> MYYGISQFSEAYNKILRNSSSHSSCQLVIFVSCLNIDALCATKMLSLLFKKQLVQSQIVPIFGYSELRRHYSQLDDNINSLLLVGFGGVIDLEAFLEIDPQEYVIDTDEKSGEQSFRRDIYVLDAHRPWNLDNIFGSQIIQCFDDGTVDDTLGEQKEAYYKLLELDEESGDDELSGDENDNNGGDDEATDADEVTDEDEEDEDETISNKRGNSSIGPNDLSKRKQRKKQIHEYEGVLEEYYSQGTTVVNSISAQIYSLLSAIGETNLSNLWLNILGTTSLDIAYAQVYNRLYPLLQDEV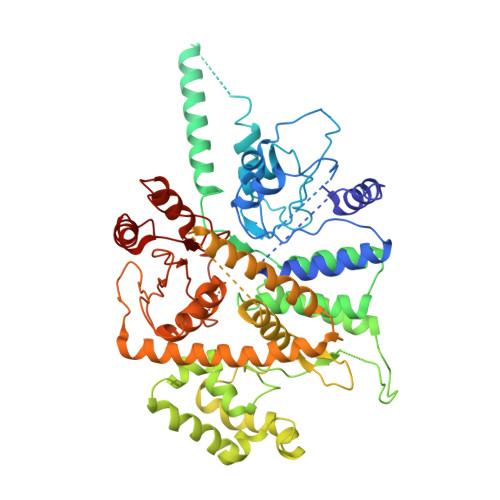KRLTPSSRNSVKTPDTLTLNIQPDYYLFLLRHSSLYDSFYYSNYVNAKLSLWNENGKKRLHKMFARMGIPLSTAQETWLYMDHSIKRELGIIFDKNLDRYGLQDIIRDGFVRTLGYRGSISASEFVEALTALLEVGNSTDKDSVKINNDNNDDTDGEEEEDNSAQKLTNLRKRWVSNFWLSWDALDDRKVELLNRGIQLAQDLQRAIFNTGVAILEKKLIKHLRIYRLCVLQDGPDLDLYRNPLTLLRLGNWLIECCAESEDKQLLPMVLASIDENTDTYLVAGLTPRYPRGLDTIHTKKPILNNFSMAFQQITAETDAKVRIDNFESSIIEIRREDLSPFLEKLTLSGLL Catabolite control protein C (CcpC) belongs to the LysR-type transcriptional regulator (LTTR) family, which regulates the transcription of genes encoding the tricarboxylic acid branch enzymes of the TCA cycle by responding to a pathway-specific metabolite, citrate. CcpC widely exists in prokaryotes and is classified as belonging to the LysR-type transcriptional regulator (LTTR) family. Two CcpC dimers interact with these sites for repression, resulting in bending of the DNA, and then blocking the access of RNA polymerase to the promoter, which results in repression of citB expression. IBD serves as a binding site of inducer and thus plays an important role in transcriptional activation by binding to inducers.

Finally, we obtained crystals for the IBD of BaCcpC and determined the crystal structure of BaCcpC-IBD in complex with citrate at 2.3 Å resolution using single-wavelength anomalous diffraction (SAD) phasing. The BaCcpC-IBD molecule is composed of two distinct regulatory domains: IBD-I (His90-Arg155 and Gly266-Gln289) and IBD-II (Asp168-Gly259). IBD-II has four β-sheets, which are surrounded by two α-helices and two 310 helices. Both the IBD-I and IBD-II subdomains adopt the typical α/β fold, which is connected by two crossover regions that form a hinge at central regions of two antiparallel β-strands (β4 and β9). Five BaCcpC-IBD molecules are in the asymmetric unit, and each molecule has an RMSD of 0.201–0.275 Å for the 144–180 Cα atoms, which emphasizes the similarity of their conformations. BaCcpC-IBD forms dimers with a head-to-tail arrangement in the asymmetric unit of its crystal structure, and both molecules have essentially the same overall structure. Superposition of two dimeric molecules in the asymmetric unit gives an RMSD of 0.327 Å for 321 Cα. The dimeric interface is stabilized by the main chain interactions Val122-Thr212* (2.82 Å, * denoting the partner molecule), Val122-Leu214* (2.92 Å), Leu124-Asp216* (2.80 Å), and Thr126-Asp216* (3.33 Å) between the β2 strand and β6 strand. The electron density corresponding to citrate molecules is found at the positively charged interface between IBD-I and IBD-II of BaCcpC-IBD. To distinguish between the terminal carboxyl groups, these were named pro-R and pro-S. The pro-R carboxyl group accepts a strong hydrogen bond from the backbone nitrogen atom of Ile100 (average distance for five molecules in the asymmetric unit: 3.12 Å). In addition, the pro-S carboxyl group also has hydrogen bonds from the side-chain NE atoms of Arg147 (2.93 Å) and Arg260 (2.80 Å). The central carboxyl group of citrate accepts hydrogen bonds from the backbone nitrogen atom of Ser129 (2.70 Å), the side-chain hydroxyl group, and Ser189 (2.59 Å) and Ser191 (2.89 Å).

>MQLQELHMLVVLAEELNMRKAAERLFVSQPALSQRLQTIEKAWGTKIFLRSQKGLTVTPAGEKIIQFANDVTDRQERIRENIDELEGEIHGTLKLAVASIIGQHWLPKVLKTYVERYPNAKVSLITGWSSEMLKSLYEDQVHIGIIRGNPEWKGRKDYLMTDHLYLVDTEISCIDDIAHTDRPFIQFKSDSTYFQEIQHWWHQKFKTSPKQTILVDQIETCKQMALHGIGYAILPSVTLEEEDKVNKMPLLDTKDHPIGRDTWLLGYEPAFELKQVQAFVSVIKDMLKQERPF[5x]>[2x]GIDPFTKTSLYESTLKNQTDLLKVTQSTVEDFRSTNQSFTRALEKDIANLPYQSL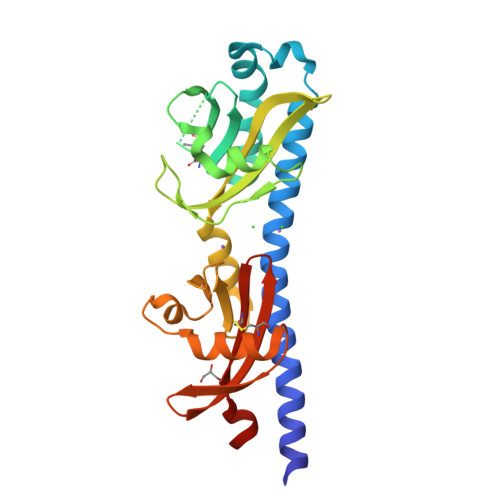ITEENIINNVGPILKYYRHSINALNVYLGLNNGKVLLSQKSNDAKMPELRDDLDIKTKDWYQEALKTNDIFVTPAYLDTVLKQYVITYSKAIYKDGKIIGVLGVDIPSEDLQNLVAKTPGNTFLFDQKNKIFAATNKELLNPSIDHSPVLNAYKLNGDNNFFSYKLNNEERLGACTKVFAYTACITESADIINKPIYKA> AHHHHHHSAALEVLFQGPGMMAKNNKTTEAKMSKKRAASEESDVEEDEDKLLSVDGLIDAEASESDEDDDEYESAVEEKESSSDKEAQDDSDDDSDAELNKLLAEEEGDGEEDYDSSEFSDDTTSLTDRLSGVKLQTIVDPNIYSKYADGSDRIIKPEINPVYDSDDSDAETQNTIGNIPLSAYDEMPHIGYDINGKRIMRPAKGSALDQLLDSIELPEGWTGLLDKNSGSSLNLTKEELELISKIQRNEQTDDSINPYEPLIDWFTRHEEVMPLTAVPEPKRRFVPSKNEAKRVMKIVRAIREGRIIPPKKLKEMKEKEKIENYQYDLWGDSTETNDHVMHLRAPKLPPPTNEESYNPPEEYLLSPEEKEAWENTEYSERERNFIPQKYSALRKVPGYGESIRERFERSLDLYLAPRVRKNKLNIDPNSLIPELPSPKDLRPFPIRCSTIYAGHKGKVRTLSIDPSGLWLATGSDDGTVRVWEILTGREVYRTTLIDDEENPDYHIECIEWNPDANNGILAVAVGENIHLIVPPIFGYDIENNGKTKIEDGFGYDTFGTVKKSNLEVNENGDGDEDGENESAKNAVKKQVAQWNKPSQKQLEKDICITISCKKTVKKLSWHRKGDYFVTVQPDSGNTSVLIHQVSKHLTQSPFKKSKGIIMDAKFHPFKPQLFVCSQRYVRIYDLSQQILVKKLLPGARWLSKIDIHPRGDNLIASSFDKRVLWHDLDLASTPYKTLRYHEKAVRSVNFHKKLPLFSSAADDGTIHVFHATVYDDMMKNPMIVPLKKLTGHKVINSLGVLDAIWHPREAWLFSAGADNTARLWTT

Erb1/Bop1 is a eukaryotic protein that was firstly described as an evolutionary conserved factor involved in large ribosomal subunit biogenesis in yeast and mammals respectively. Its function is essential in the processing of rRNA precursors that give rise to the mature 5.8S and 25/28S particles. Erb1 directly interacts with Nop7 and Ytm1 proteins (Pes1 and Wdr12 in mammals, respectively) forming Nop7 sub-complex (called PeBoW in mammals) that co-purifies with pre60S particles but remains stable even after its dissociation from pre-ribosomes. The C-terminal region of Erb1 was predicted to contain seven WD repeats that form a β-propeller domain of unclear function.

Here we present the structure of the β-propeller domain of Erb1 at 1.6Å resolution that was obtained during crystallization trials of Erb1/Nop7 dimer. The solved structure of the C-terminal domain of Erb1 has confirmed that it folds into a seven-bladed β-propeller as previously predicted. Structure analysis led us to slightly extend exact boundaries of the domain (residues 427–807) towards the N-term, when compared to the sequence-based prediction (residues 435–807) because the strand D (outermost) of blade 7 (most C-terminal) is actually formed by residues 427–433 which participate in the “velcro-like” closure of the domain. Electron density map allowed us to trace and build model for residues 515–534 and 571–594, being the rest of the insertion unmodeled. Helix H2 (residues Tyr520-Asp532) appears between strands 2C and 2E and is attached to the base of the propeller. We observe that in this case there is a different interaction network, conserved in Erb1/Bop1 family but not in other WD repeat-containing proteins, that involves strand 2D from blade 1 and a short α-helix, H3, from blade 2 (Gln580-Lys585). The third area corresponds to the long 6C-7D loop which forms an important extension and introduces Asp757, Met758 and Met759 into a cavity formed between Phe635, Tyr665 and Gln670 from blades 3 and 4. Indeed, as seen for the electrostatic surface analysis, the tool found a big region of basic residues on the surface that included five blades and the entrance to the central channel on the top face of the propeller. Taken together, our observations demonstrate that the C-terminal domain of Erb1 is likely to form part of a protein complex and is capable of binding RNA unspecifically through a defined surface.>GPLGSSYSMEQVEGITSEYIVKNADMFAVAVSLVSGKILYISNQVASIFHCKKDAFSDAKFVEFLAPHDVSVFHSYTTPYKLPPWSVCSGLDSFTQECMEEKSFFCRVSVGKHHENEIRYQPFRMTPYLVKVQEQQGAESQLCCLLLAERVHSGYEAPRIPPEKRIFTTTHTPNCLFQAVDERAVPLLGYLPQDLIETPVLVQLHPSDRPLMLAIHKKILQAGGQPFDYSPIRFRTRNGEYITLDTSWSSFINPWSRKISF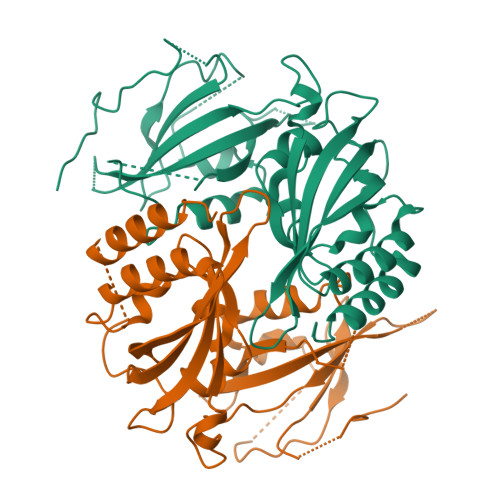IIGRHKVRVGPLNEDVFAAPPCPEEKTPHPSVQELTEQIHRLLMQPVP[2x]>MGSSHHHHHHSQDPMLSKDIIKLLNEQVNKEMNSSNLYMSMSSWCYTHSLDGAGLFLFDHAAEEYEHAKKLIIFLNENNVPVQLTSI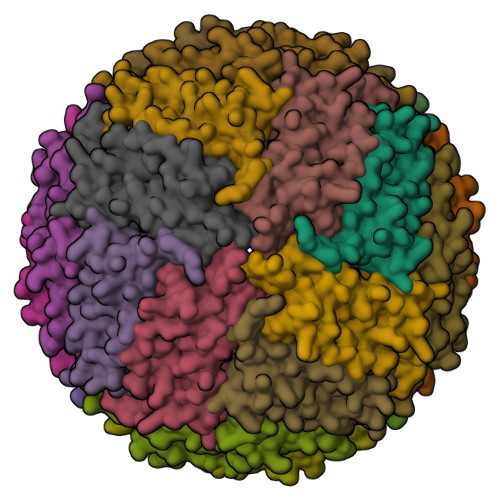SAPEHKFEGLTQIFQKAYEHEQHISESINNIVDHAIKSKDHATFNFLQWYVAEQHEEEVLFKDILDKIELIGNENHGLYLADQYVKGIAKSRKS[6x]>[10x]ADQPIDADVTVIGSGPGGYVAAIKAAQLGFKTVCIEKNETLGGTCLNVGCIPSKALLNNSHYYHMAHGTDFASRGIEMSEVRLNLDKMMEQKSTAVKALTGGIAHLFKQNKVVHVNGYGKITGKNQVTATKADGGTQVIDTKNILIATGSEVTPFPGITIDEDTIVSSTGALSLKKVPEKMVVIGAGVIGVELGSVWQRLGADVTAVEFLGHVGGVGIDMEISKNFQRILQKQGFKFKLNTKVTGATKKSDGKIDVSIEAASGGKAEVITCDVLLVCIGRRPFTKNLGLEELGIELDPRGRIPVNTRFQTKIPNIYAIGDVVAGPMLAHKAEDEGIICVEGMAGGAVHIDYNCVPSVIYTHPEVAWVGKSEEQLKEEGIEYKVGKFPFAANSRAKTNADTDGMVKILGQKSTDRVLGAHILGPGAGEMVNEAALALEYGASCEDIARVCHAHPTLSEAFREANLAASFGKSINF;>[5x]GEHIPGTLRFR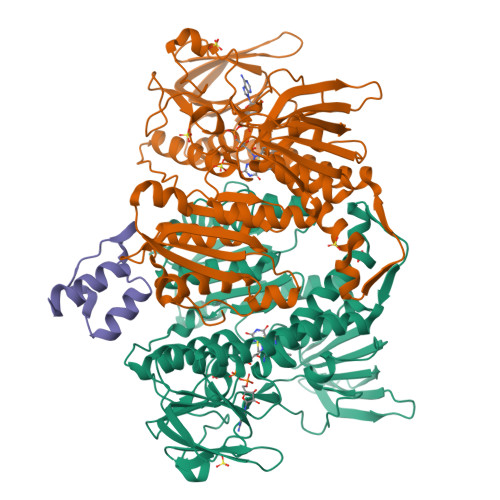LSPAARNILEKHSLDASQGTATGPRGIFTKEDALKLVQLKQTGKILEHHHHHH>[2x]PSSSMADFRKFFAKAKHIVIISGAGVSAESGVPTFRGAGGYWRKWQAQD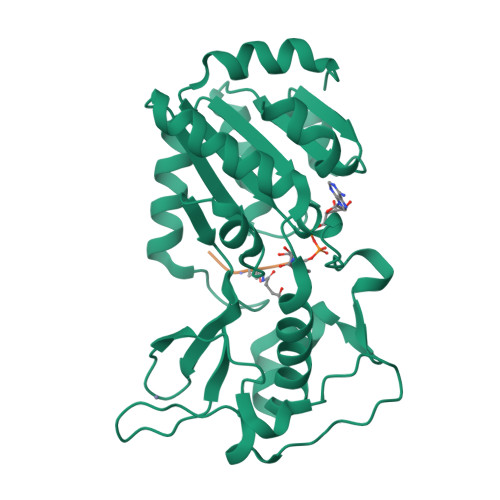LATPLAFAHNPSRVWEFYHYRREVMGSKEPNAGHRAIAECETRLGKQGRRVVVITQNIDELHRKAGTKNLLEIHGSLFKTRCTSCGVVAENYKSPICPALSGKGAPEPGTQDASIPVEKLPRCEEAGCGGLLRPHVVWFGENLDPAILEEVDRELAHCDLCLVVGTSSVVYPAAMFAPQVAARGVPVAEFNTETTPATNRFRFHFQGPCGTTLPEALA>[6x]MGSSHHHHHHSSGLEVLFQGPAERISKQSTPFVGAQIFIEPGQTQEQIEQWFKLLAESNMTTCRIRMFGKYMKTPSGTYDFTLFDRAFKLADKYHIKVYATLFPDTEFTDVGGFKFPHSREHQKEVEDYIKNVVSHFSQYKNLAAWVLINEPGTPNLPFNEPFTKERFSDWKKEHNFSEYNEKGYPVLNFEKENFIIDYHNWYLNWLANQVRLYDKQHDLHVNPHNVFKLSGLYDFPTWRTFLNSLGGSAHASWHFGYFPRKAYTVAMSANAELIRSGAGELPWLMTELQGGNNLYSGANPLCPTAEEIIQWLWINFATEAKGGIFWSFNARSTAAEAGEWAMINFKNKSSDRLIAAATIGKFITENVKMMSNIKTLNSGISILYNHESMWVEAAQTRGKLNGNGRSIGAVMCSPLSYFEALSETGLQANFKEIKEFDFSLNDYTDQVIILSHQIALDNKVIKQLESFVEKGGTLI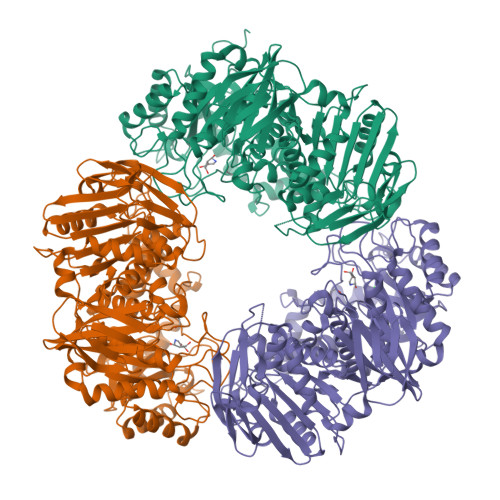ADGLTGYYDYQAHSTVVSGFALENLFGSYPIEYKIKENLFSLDFEKDNYKLPAHLWKGTIETSKATPIMDKEGECIACINQYGKGKVFWIPSPIALGARESKDFSELSKLTVSLLPNKILNDNPHFDKHYKDVMMKSFKSNGTMYSLIINKSASVQTVDIVGGKGKAFILFANKNAHSTANKLTISPEETVIIKWKNN1-{(1S)-1-[4-(3-amino-1H-indazol-6-yl)-5-chloro-1H-imidazol-2-yl]-2-phenylethyl}-3-[5-chloro-2-(1H-tetrazol-1-yl)benzyl]urea 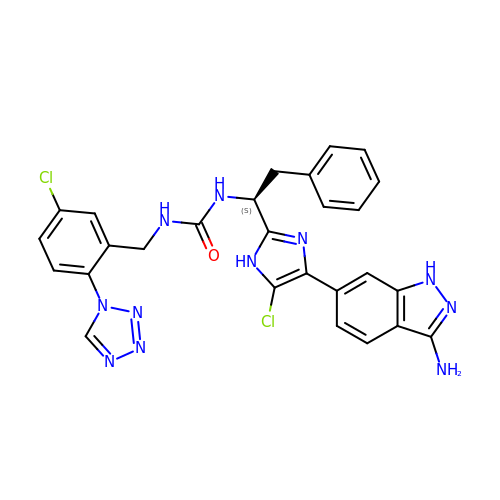| C27 H23 Cl2 N11 O | LCVIWSIVTGTOCS-NRFANRHFSA-N> GAACGACACTGA;> CGTCGACTC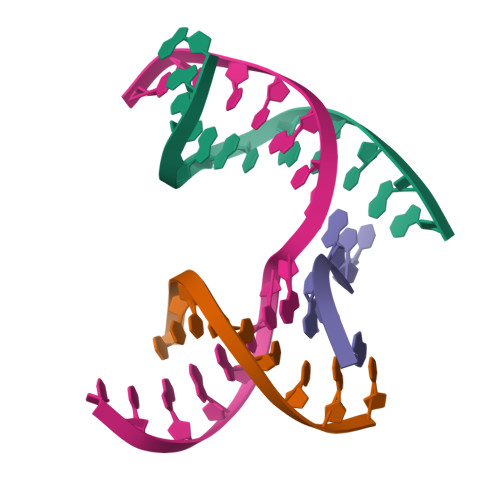;> TCAACG;> TCGAGTCGGTGTCGT> MTTLTRQDLNSAQVVADVLSEFLEVAVHLILYVREVYPVGIFQKRKKYNVPVQMSCHPELNQYIQDTLHCVKPLLEKNDVEKVVVV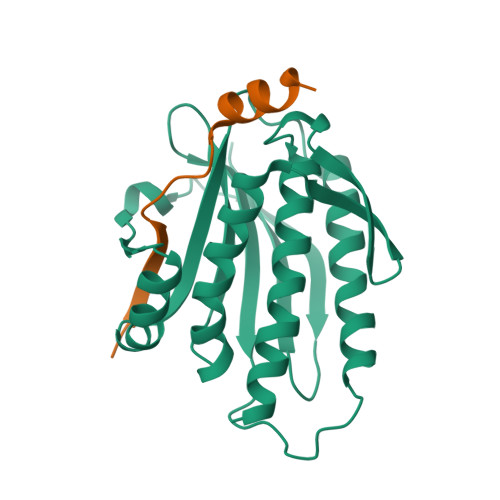ILDKEHRPVEKFVFEITQPPLLSINSDSLLSHVEQLLRAFILKISKVDKVLDHNPPGCTFTVLVHTREAATRNMEKIQVIKDFPWILADEQDVHMHDPRLIPLKTMTSDILKMQLYVEERAHKNS;> MGDKKIVIMPCKCAPSRQLVQVWLQAKE>[4x]EAPYASLTEIEHLVQSVCKSYRETCQ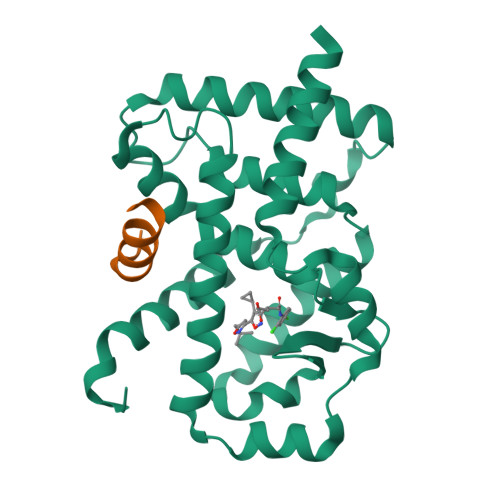LRLEDLLRQRSNIFSREEVTGYQRKSMWEMWERCAHHLTEAIQYVVEFAKRLSGFMELCQNDQIVLLKAGAMEVVLVRMCRAYNADNRTVFFEGKYGGMELFRALGCSELISSIFDFSHSLSALHFSEDEIALYTALVLINAHRPGLQEKRKVEQLQYNLELAFHHHLCKTHRQSILAKLPPAGKLASLCSQHVERLQIFQHLHPIVVQAAFPPLYKELFSTETESPVGLSK;>[4x]TNMGLEAIIRKALMGKYDQWEE>[7x]MAGPEPLAALPDGDLLDFLLNDDAPAAGSPAGDGPLLGDWVLPELELLDKEMDSFISSLLSPSEDEPCLL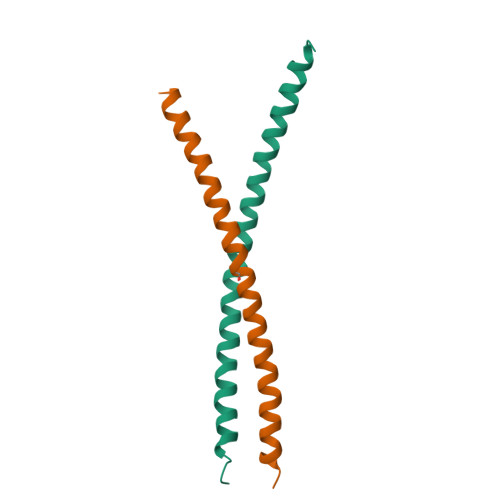QGCLPADSDSSTSEDQNPFHSSGSDVASSPQSSDIVQFDHNYSLHQDWPALESVRSDMAEGDVSIDLETWMCLEGTNETLQESCSFPVTVAVDAGPQLMPGAPMQSNFPELVLTEEERQLLEKDGVSLPTCLPLTKAEERLLKKVRRKIRNKQSAQDSRRRKKIYVDGLENRVAACTAQNHELQKKVQLLQKQNMSLLEQLRKLQALVRQSTTKTTTASTCIMVLVLSFCLILSPSLYSFGSRGPQPEFRVLSRQIREFPNKVWQAAPAVQEEVVLERLSPEPEDTSLGSLNQSREEGQSPPKPDPRSAFNGNSSSDPPAGSELGHPQPQEQQSRRDALHSEVLAPWKDENQEWVERTTSVVIQQHRTDEM(1R,2R)-N-(2-AMINOETHYL)-2-{[(4-METHOXYPHENYL)SULFONYL]METHYL}CYCLOHEXANECARBOXAMIDE | C17 H26 N2 O4 S | 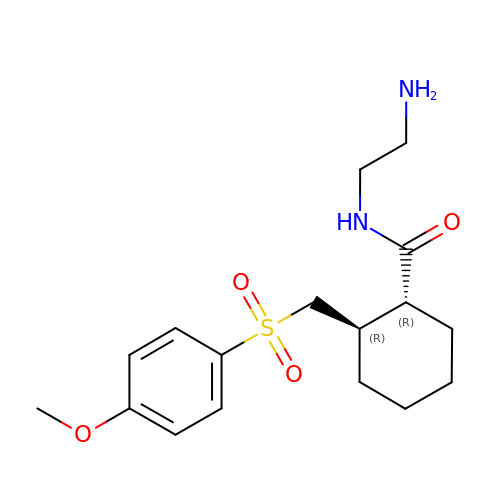QTGNVZPFJQOWFL-XJKSGUPXSA-N> GSHMMLSLNNLQNIIYNPVIPFVGTIPDQLDPGTLIVIRGHVPSDADRFQVDLQNGSSMKPRADVAFHFNPRFKRAGCIVCNTLINEKWGREEITYDTPFKREKSFEIVIMVL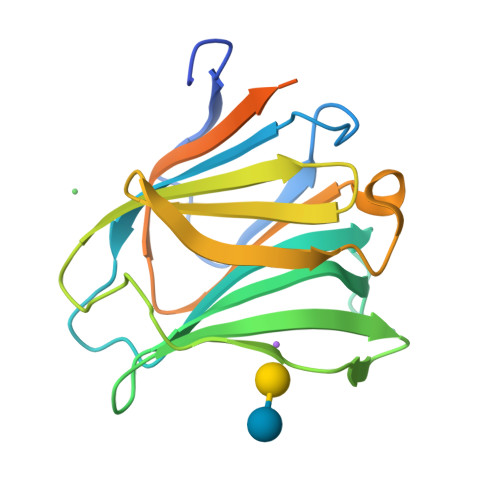KDKFQVAVNGKHTLLYGHRIGPEKIDTLGIYGKVNIHSIGFSFSSDLQSTQASSLELTEISRENVPKSGTPQLRLP> ASKAAAPPPVRLFGVEGTYATALYQAAAKNSSIDAAFQSL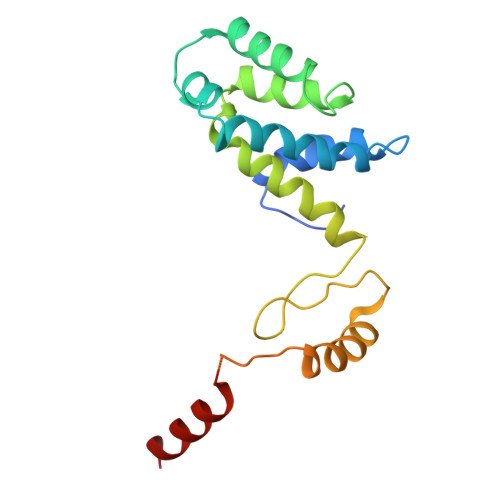QKVESTVKKNPKLGHLLLNPALSLKDRNSVIDAIVETHKNLDGYVVNLLKVLSENNRLGCFEKIASDFGVLNDAHNGLLKGTVTSAEPLDPKSFKRIEKALSASKLVGQGKSLKLENVVKPEIKGGLIVELGDKTVDLSISTKIQKLNKVLEDSI> QAQITGRPEWIWLALGTALMGLGTLYFLVKGMGVSDPDAKKFYAITTLVPAIAFTMYLSMLLGYGLTMVPFGGEQNPIYWARYASWLFTTP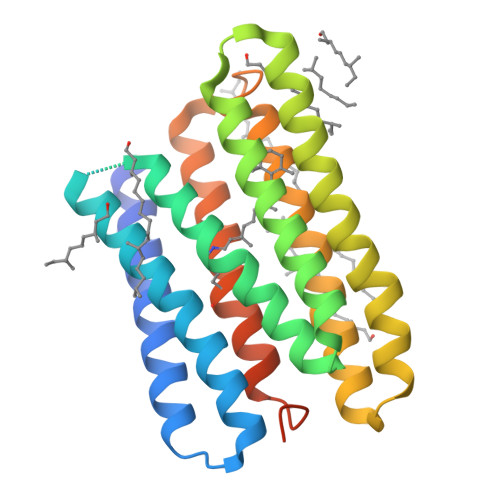LLLLDLALLVDADQGTILALVGADGIMIGTGLVGALTKVYSYRFVWWAISTAAMLYILYVLFFGFTSKAESMRPEVASTFKVLRNVTVVLWSAYPVVWLIGSEGAGIVPLNIETLLFMVLDVSAKVGLGLILLRSRAIFGEAEAPEPSAGDGAAATSD Like Plks, Cdc5 contains a Ser/Thr kinase domain followed by a polo-box domain that mediates substrate recognition and sub-cellular localization. The polo-box domain is made up of two polo boxes that together define the p(S/T)-binding pocket. Cdc5 promotes the release of Cdc14 from the nucleolus and regulates the mitotic exit network (MEN)9,16–18 as well as cytokinesis. Here we demonstrate that the polo-box domain of Cdc5 uses distinct surfaces to bind phosphorylated and non-phosphorylated substrates.

To confirm how Cdc5 recognizes phosphorylated substrates, we then solved the structure of Cdc5 bound to a phosphorylated peptide derived from the spindle-pole body protein Spc72 (Spc72P, 227SLAQSpSPAGSQ237). As expected, the Spc72P phosphopeptide bound along the groove determined by the two polo-boxes and adopts an extended conformation that runs antiparallel to β1, effectively extending the β-sheet of the first polo-box by one strand. The strictly conserved His641 and Lys643 cradle the phosphate group, confirming that Cdc5 recognizes phosphorylated substrates the same way as other Plk1 homologs. As expected, the Spc72 peptide bound to the groove at the interface of the two polo boxes. Using isothermal calorimetry, we confirmed that the Spc72P peptide interacted with the polo-box domain of Cdc5, and the interaction was phosphorylation dependent. We found that Spc72P bound to Cdc5 and Cdc5-Dbf4 with similar affinities. In vitro, Dbf4 and phosphorylated peptides can bind simultaneously and not competitively to the polo-box domain of Cdc5.

>GALSPGGTKQKYKEVVDIEAQRRLNDLAREARIRRAQQAVLRKELIATSTNVIKSEISLRILASECHLTLNGIVEAEAQYKMGGLPKSRLPKIKHPMIVTKWVDYSNKHGFSYQLSTEDIGVLFNNGTTVLRLADAEEFWYISYDDREGWVASHYLLSEKPRELSRHLEVVDFFAKYMKANLSRVSTFGREEYHKDDVFLRRYTRYKPFVMFELSDGTFQFNFKDHHKMAISDGGKLVTYISPSHESTTYPLVEVLKYGEIPGYPESNFREKLTLIKEGLKQKSTIVTVD[2x];>[2x]SLAQSSPAGSQ>MHHHHHHHHHHHHLPPITPQELESMSPQEQRAALGDRLFLKVYEIAPELAPKITGMFLEMKPKEAYELLN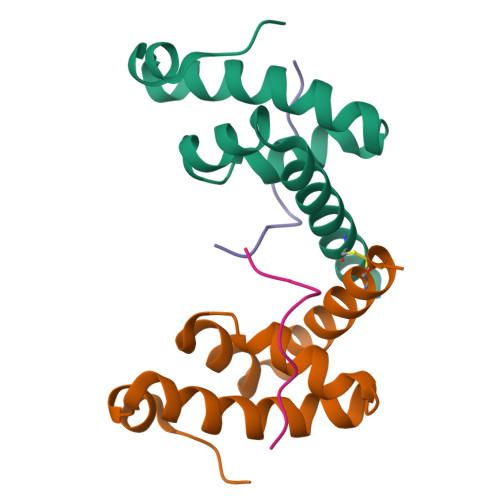DQKRLEERVTEALCVLKAHQTA[2x];>HHMNPNATEFMPGR[2x]>SSKSCLVARIQLLNNEFVEFTLSVESTGQESLEAVAQRLELREVTYFSLWYYNKQNQRRWVDLEKPLKKQLDKYALEPTVYFGVVFYVPSVSQLQQEITRYQYYLQLKKDILEGSIPCTLEQAIQLAGLAVQADFGDFDQYESQDFLQKFALFPVGWLQDEKVLEEATQKVALLHQKYRGLTAPDAEMLYMQEVERMDGYGEESYPAKDSQGSDISIGACLEGIFVKHKNGRHPVVFRWHDIANM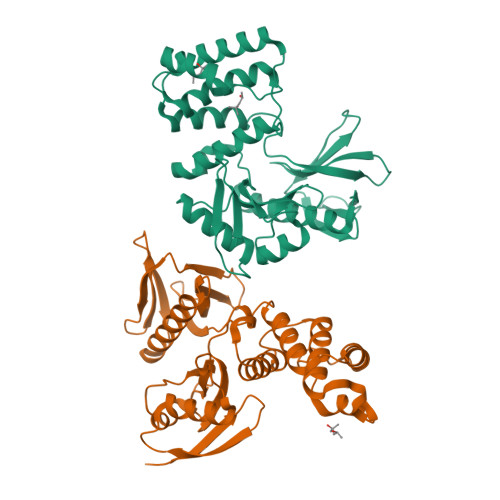SHNKSFFALELANKEETIQFQTEDMETAKYIWRLCVARHKFYRLNQCNLQTQTVTV[2x]> MADIGSEFYTLNWQPPYDWSWMLGFLAARAVSSVETVADSYYARSLAVGEYRGVVTAIPDIARHTLHINLSAGLEPVAAECLAKMSRLFDLQCNPQIVNGALGRLGAARPGLRLPGCVDAFEQGVRAILGQCVSVAMAAKLTARVAQLYGERLD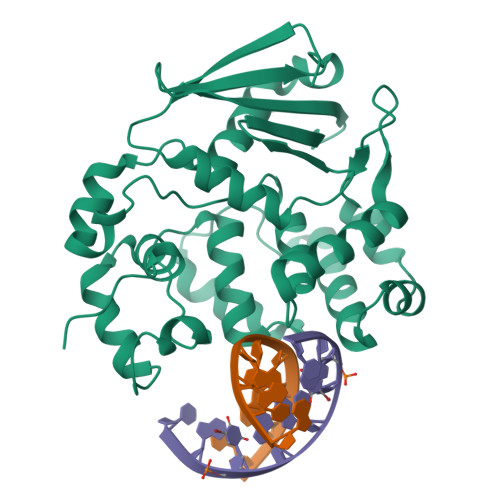DFPEYICFPTPQRLAAADPQALKALGMPLKRAEALIHLANAALEGTLPMTIPGDVEQAMKTLQTFPGIGRWTANYFALRGWQAKDVFLPDDYLIKQRFPGMTPAQIRRYAERWKPWRSYALLHIWYTEGWQPDEA>KALFQPLTPGSREFEDVVNILHSSYLEPTSVTNFNYRRACLVHNELLEKEFTEKRRELKFDGRLDKELSESYAFLMVDRYQVQTICEKGLHVGQSKITILGSPSMGVYLSRYADLLQANPLDTGAMGDVVIFKIMKGKIKSIYDPMGVKSLDPTPKHECHVSKNANRITSLLAYRAYELTQYYFYEYGF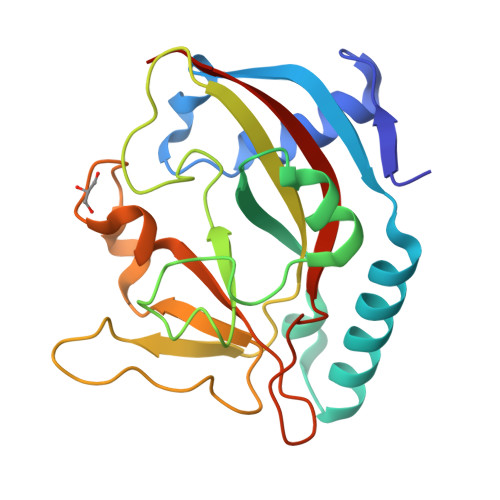DELRRRPRHVCPYAVVSFTYKDDIQ[2x]> G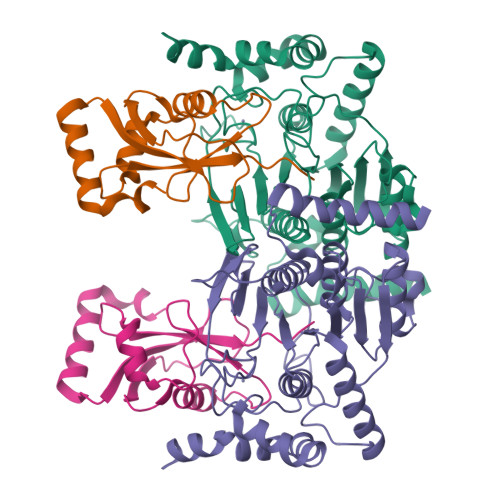PHMLKIADQSVDLNLKLMKWRILPDLNLDIIKNTKVLLLGAGTLGCYVSRALIAWGVRKITFVDNGTVSYSNPVRQALYNFEDCGKPKAELAAASLKRIFPLMDATGVKLSIPMIGHKLVNEEAQHKDFDRLRALIKEHDIIFLLVDSRESRWLPSLLSNIENKTVINAALGFDSYLVMRHGNRDEQSSKQLGCYFCHDVVAPTDSLTDRTLDQMCTVTRPGVAMMASSLAVELMTSLLQTKYSGSETTVLGDIPHQIRGFLHNFSILKLETPAYEHCPACSPKVIEAFTDLGWEFVKKALEHPLYLEEISGLSVIKQEVERLGNDVFEWEDDESDEIA;> GPHMKSTFKSEYPFEKRKAESERIADRFPNRIPVICEKAEKSDIPEIDKRKYLVPADLTVGQFVYVIRKRIMLPPEKAIFIFVNDTLPPTAALMSAIYQEHKDKDGFLYVTYSGENTFG> NALL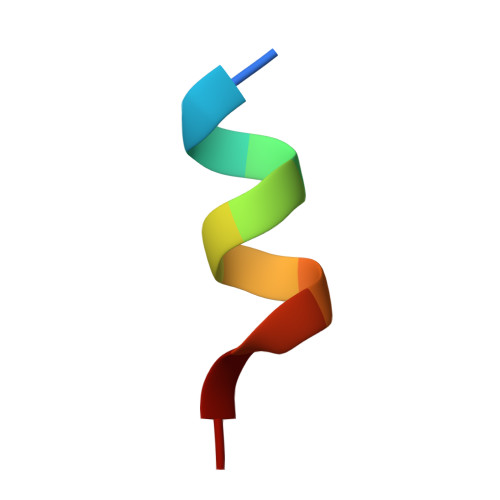RYLLDKD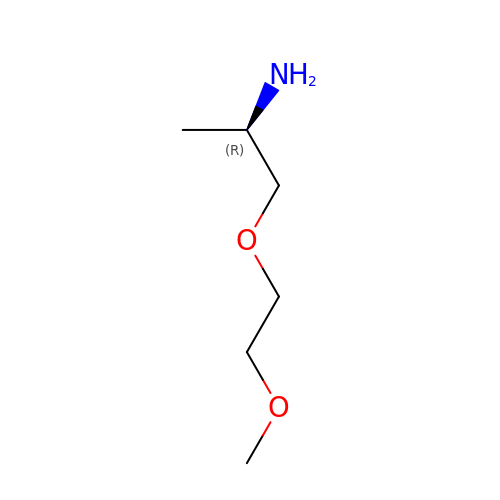(2~{R})-1-(2-methoxyethoxy)propan-2-amine | C6 H15 N O2 | CMXIILNXYHCYPP-ZCFIWIBFSA-N> GPLGSEILRHSMDPATFTFNFNNEPWVRGRHETYLCYEVERMHNDTWVKLAQRRGFLANQAKHKHGFLEGRHAELCFLDVIPFWKLDLDQDYRVTCFTSWSPCFSCAQEMAKFISKNKHVSLCIKTARIYDDKGRAAEGLRTLAEAGAKISIMTYSEFKHCWDTFVDHQGAPF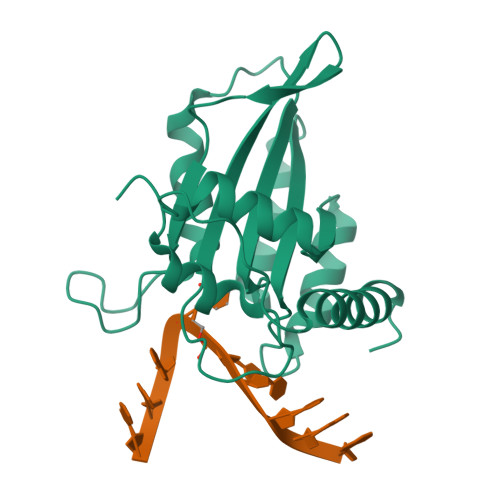QPWDGLDEHSQDLSGRLRAILQNQEN>[4x]VASNNVNDLITVTKQTIKVGDGKDNVAAAHDGKDIEYDTEFTIDNKVKKGDTMTINYDKNVIPSDLTDKNDPIDITDPSGEVIAKGTFDKATKQITYTFTDYVDK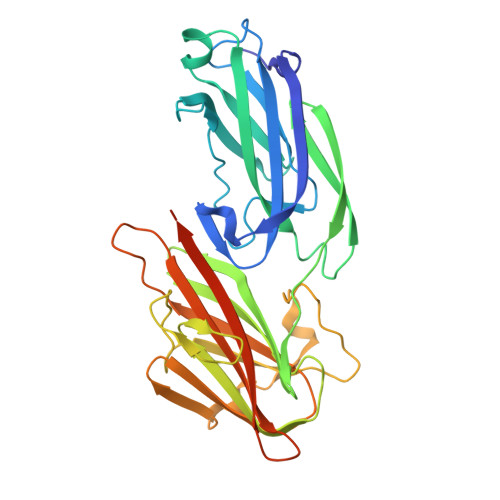YEDIKARLTLYSYIDKQAVPNETSLNLTFATAGKETSQNVSVDYQDPMVHGDSNIQSIFTKLDENKQTIEQQIYVNPLKKTATNTKVDIAGSQVDDYGNIKLGNGSTIIDQNTEMKVYKVNPNQQLPQSNRIYDFSQYEDVTSQFDNKKSFSNNVATLDFGDINSAYIIKVVSKYTPTSDGELDIAQGTSMRTTDKYGYYNYAGYSNFIVTSNDTGGGDGTVKPELEHHHHHH Building on the previously established methods in assembling enterovirus RdRP EC and in capturing various EC states, we used an EV71 RdRP bearing a C291M mutation in such approaches, since the equivalent PV RdRP mutant (C290M) was shown to produce higher quality EC crystals. Building on our recent work reporting an enterovirus 71 (EV71) RdRP EC with an intermediate conformation of its template-product duplex, here we report three types of translocation intermediate crystal structures that define multiple nucleic acid conformations bridging the pre- and post-translocation states, both in the regulate forward translocation and in an unusual reverse translocation induced by pyrophosphate (PPi) and divalent metal ions. These structural data, in combination with enzymology characterization of the RdRP, highlight the key role of RdRP motif G in controlling the critical movement of the template RNA strand that is probably the rate-limiting step for both forward and reverse translocations. A striking common feature for both modes of translocation is that the template backbone, in particular for positions −2 to +1, stayed fixed relative to its starting point of translocation. As we pointed out previously, this phenomenon is probably related to two motif G residues (T114-S115 in EV71 RdRP, “G” symbol in Figs. 2d and 3d) that create a hurdle-like steric blockage right at the +1/+2 junction of the template backbone.

Among these mutants, a class II mutant T114S-S115T (abbreviated as ST) yielded EC crystals that are suitable for structure determination. This mutant has a kcat value comparable to the WT but its KM,NTP is about 50-fold of the WT level. The much lower NTP affinity could indicate the alteration of the catalytic pocket at the NTP binding stage. Interestingly, the ST mutant-derived EC structure indeed exhibited a previously unidentified conformation with the −2 to +2 template nucleotides clearly occupying intermediate positions, while the product strand almost reached the post-translocated position (Table 1 and Fig. 5, S6M (C0) structure, 2.1 Å resolution, C0 indicates that the intermediate state is in an NAC prior to the corresponding post-translocation state of this native EC). Although the nearly full-register movement of product strand had vacated the active site, we did not observe NTP-like electron densities in it, and therefore the incoming NTP-assisted translocation is not evident. Previously determined native enterovirus EC crystal structures all adopted the post-translocation conformation, and therefore it is probable that the hurdle residue mutation relatively destabilize the post-translocation state, allowing the capture of the observed intermediate state. Comparing to the pre-translocation state, the template +1 phosphate moved by 2.2 Å toward the upstream and residue 115 backbone amide nitrogen interacting with the phosphate oxygen also moved 1.7 Å accordingly.

> GEIQWVKPNKETGRLNINGPTRTKLEPSVFHDVFEGNKEPAVLHSKDPRLEVDFEQALFSKYVGNTLYEPDEYIKEAALHYANQLKQLDIDTSQMSMEEACYGTENLEAIDLHSTAGYPYSALGIKKRDILDSTTRDVSKMKFYMDKYGLDLPYSTYVKDELRSIDKIKKGKSRLIEASSLNDSVYLRMTFGHLYETFHANPGTVTGSAVGCNPDTFWSKLPILLPGSLFAFDYSGYDASLSPVWFRALELVLREIGYSEEAVSLVEGINHTHHVYRNKTYCVLGGMPSGMSGTSIFNSMINNIIIRALLIKTFKGIDLDELNMVAYGDDVLASYPFPIDCLELARTGKEYGLTMTPADKSPCFNEVNWDNATFLKRGFLPDEQFPFLIHPTMPMKEIHESIRWTKDARNTQDHVRSLCLLAWHNGKQEYEKFVSAIRSVPVGKALAIPNYENLRRNWLELFHHHHHH>[5x]MARGLVIGEALIDIVDGPDPAEYVGGSPLNVAVGLARLGRDVDLLTHIGRDARGRRIAEYIESSGVQLVSGSQTADRTPTATARIGPDGSATYAFDLEWQIPDTPPVTPPLLVHTGSIAAAREPGCLAVAALLDAYRAAATVSFDPNVRPSLSADPDLTRERIQRLVERSDIIKASAEDLHWIDPTQPPEQTARAWLACGPAIVALTLGDQGAVAFCAAGPASVPAQPVRVVDTVGAGDAFMAGLLDTLWEQGLLGADRRTELRKIGVSALTSALEVAALTSALTVARAGADLPYRADLRQSR;> MARGLVIGEALIDIVDGPDPAEYVGGSPLNVAVGLA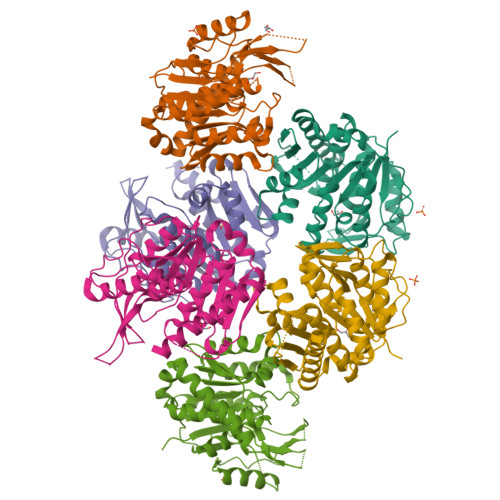RLGRDVDLLTHIGRDARGRRIAEYIESSGVQLVSGSQTADRTPTATARIGPDGSATYAFDLEWQIPDTPPVAPPLLVHTGSIAAAREPGCLAVAALLDAYRAAATVSFDPNVRPSLSADPDLTRRRIQRLVERSDIIKASAEDLHWIDPTQPPEQTARAWLACGPAIVALTLGDQGAVAFCAAGPASVPAQPVRVVDTVGAGDAFMAGLLDTLWEQGLLGADRRTELRKIGVSALTSALEVAALTSALTVARAGA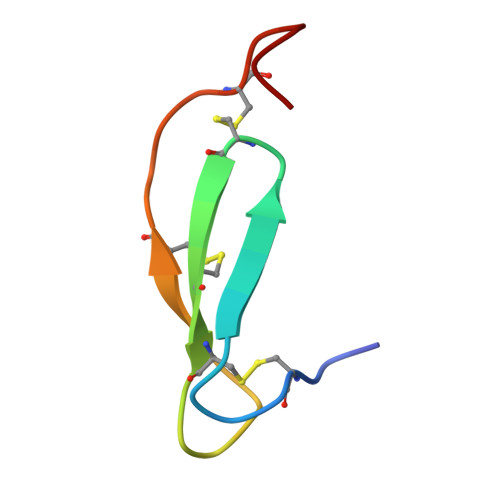> GSSCTPGATFRNRCNTCRCGSNGRSASCTLMACPPGSY(2S)-6,8-dichloro-2-(trifluoromethyl)-2H-chromene-3-carboxylic acid | C11 H5 Cl2 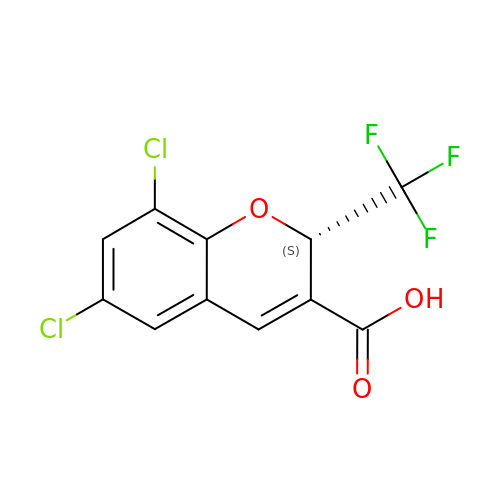F3 O3 | ZFKBWSREWJOSSJ-VIFPVBQESA-N>[5x]SNADWLTLNVGGRYFTTTRSTLVNKEPDSMLAHMFKDKGVW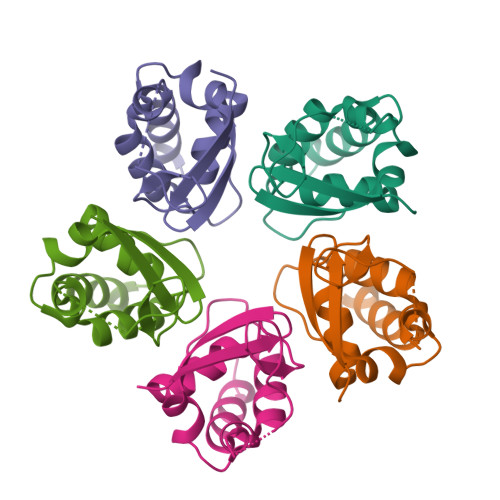GNKQDHRGAFLIDRSPEYFEPILNYLRHGQLIVNDGINLLGVLEEARFFGIDSLIEHLEVAIKNS> ETGESPPVFIKKPVDQIGVSGGVASFVCQATGDPKPRVTWNKKGKKVNSQRFETIEFDESAGAVLRIQPLRTPRDENIYECVAQNPHGEVTVHAKLTVLREDQLPPGFPNIDMGPQLKVVERTRTATMLCAASGNPDPEITWFKDFLPVDPSTSNGRIKQLRSGGLQIESSEETDQGKYECVASNSAGVRYSSPANLYVRVRRVAPRFSILPVSHEIMPGGNVNITCVAVGSPMPYVKWMQGAEDLTPEDDMPVGRNVLELTDVKDSANYTCVAM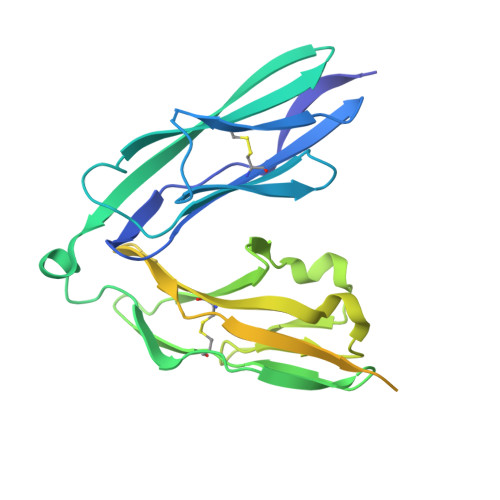SSLGVIEAVAQITVKSKGHHHHHH> GSHMSNTQTVL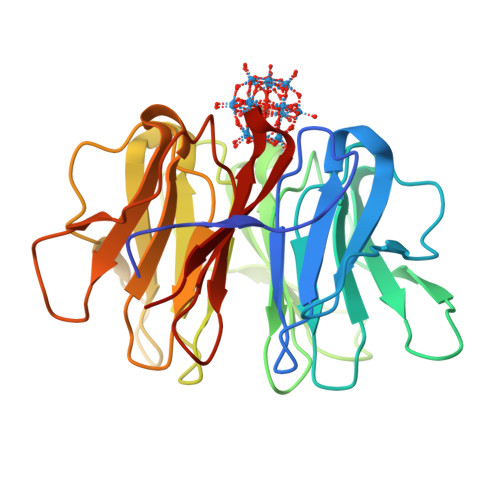PFTGLNTPNGVAVDSAGTVYVTDHGNNRVVKLAAGSNTQTVLPFTGLNTPSGVAVDSAGTVWVTDHGNNRVVKLAAGSNTQTVLPFTGLNTPNGVAVDSAGTVYVTDHGNNRVVKLAAGSNTQTVLPFTGLNTPSGVAVDSAGTVWVTDHGNNRVVKLAAGSNTQTVLPFTGLNTPNGVAVDSAGTVYVTDHGNNRVVKLAAGSNTQTVLPFTGLNTPSGVAVDSAGTVWVTDHGNNRVVKLAAG> MHHHHHHLILAPMVRVGTLPMRLLALDYGADIVYCEELIDLKMIQCKRVVNEVLSTVDFVAPDDRVVFRTCEREQNRVVFQM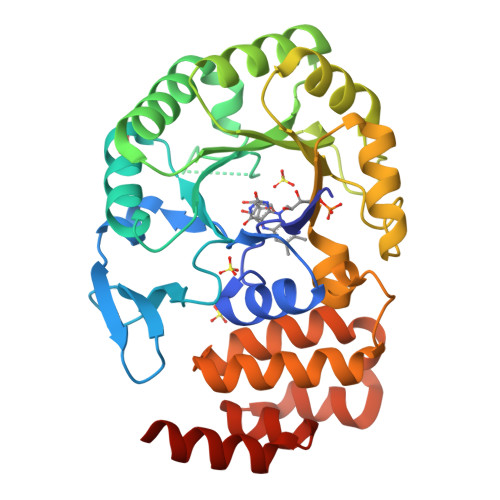GTSDAERALAVARLVENDVAGIDVNMGCPKQYSTKGGMGAALLSDPDKIEKILSTLVKGTRRPVTCKIRILPSLEDTLSLVKRIERTGIAAIAVHGRKREERPQHPVSCEVIKAIADTLSIPVIANGGSHDHIQQYSDIEDFRQATAASSVMVARAAMWNPSIFLKEGLRPLEEVMQKYIRYAVQYDNHYTNTKYCLCQMLREQLESPQGRLLHAAKSSREICEAFGLGAFYEETTQELDAQQAR We show here that when long wavelengths are combined with the Mesh&Collect data-collection approach and when a genetic algorithm (GA) is used to compile a data set, a native SAD experiment can yield a structure solution from microcrystals. Furthermore, the GA algorithm can effectively generate a highly complete data set from hundreds of naturally multi-oriented samples collected at long wavelength, thus permitting the compilation of a highly complete data set with high multiplicity, and thus preserving a weak anomalous signal and enabling structure solution by standard SAD phasing procedures. In summary, Mesh&Collect data collection using softer X-rays extends SAD phasing from naturally occurring anomalous scatterers to micrometre-sized crystals.

Data were collected to the maximum resolution possible of 1.929 Å owing to the geometry of the camera and the wavelength. The data collection (30 grid scans for 298 partial data sets) was completed within 2 h. The autoprocessing routines could index and integrate 180 partial data sets out of the 298 that were collected. The aggregated data set, obtained from the merging of 116 partial data-set wedges, resulted in high overall completeness and decent data quality, which allowed the location of the anomalous scatterers, successful phasing and structure refinement using standard methodology. SHELXD correctly determined the Ca2+ and Mn2+ ions and the S atoms at the Met42 and Met129 sites, producing CCall, CCweak and PATFOM values of 34.2, 21.7 and 55.8, respectively. The anomalous difference Fourier map peak heights were 46σ for Mn2+, 27σ for Ca2+, 7.5σ for the Met129 SD atom and 6.3σ for the Met42 SD atom, as assigned using ANODE. A best weighted mean phase error (wMPE) of 34° and a CC for the partial model of 22% were obtained in SHELXE, with 119 amino acids automatically built. Cullis values calculated starting from the Ca2+ ion or the Mn2+ ion alone were 0.90 and 0.89, respectively, indicating that in the case of proteins of analogous size but lacking cysteines or methionines a Ca2+ ion or the Mn2+ ion alone could provide significant phasing information. Finally, no evidence of radiation damage was present in the electron-density maps for the crystal structure of ConA.

> ADTIVAVELDTYPNTDIGDPSYPHIGIDIKSVRSKKTAKWNMQNGKVGTAHIIYNSVDKRLSAVVSYPNADSATVSYDVDLDNVLPEWVRVGLSASTGLYKETNTILSWSFTSKLKSNSTHETNALHFMFNQFSKDQKDLILQGDATTGTDGNLELTRVSSNGSPQGSSVGRALFYAPVHIWESSAVVASFEATFTFLIKSPDSHPADGIAFFISNIDSSIPSGSTGRLLGLFPDAN>[12x]MAITPEQIAVEYPIPTYRFVVSVGDEQIPFNNVSGLDVHYDVIEYKDGIGNYYKMPGQRQSINITLRKGVFPGDTKLFDWINSIQLNQVEKKDIAISLTNEAGTEILMTWNVANAFPTSFTSPSFDATSNEIAVQEIALTADRVTIQAA;>MTTIT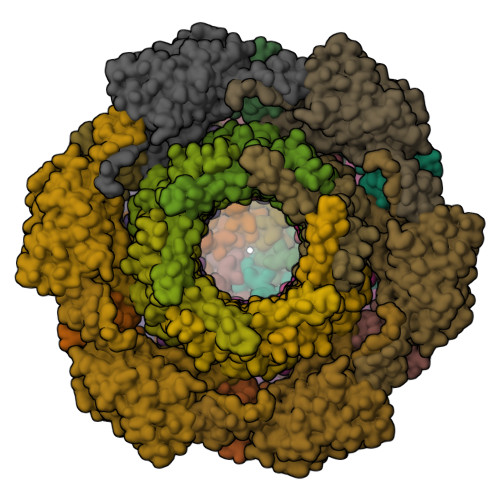TYPGVYIEEDASLSLSVSSSATAVPVFAVAGDNPLISGKPYIRISNWLEYLTLKNEQFDPANTLDISLRAYFINGGGYCYLVQTTDLEKQVPKLDDVTLLVAAGENITTAVSTLCKPGKGLFAIFDGPTTELKSDGTSNSDYDPNPFAAVYYPWLTADWTTTIDIPPSAAIAGVYCSVDSTRGVWKAPANVPIQGGLQPKYPVTDDLQAQYNQGKALNMIRTFPKSGTLVWGARTLEDNDNWRYIPVRRLFNSAERDIKNAMSFAVFEPNSQPTWERVRSAVNNYLYSLWQQGGLAGNKPDDAYFVQIGKDITMTDDDIKQGKMIIKIGMAAVRPAEFIILQFTQNTAQ[6x];>[6x]MTIIIASDNAIIEINQALNTILSQYLNITGQNIDIRFDLPEINSIQSEPTVSVFLYEIHEDLQLRSAESRRYNPSTNTLLPGWVNINCNYLITYWDASKPSSDSSSPDSQPNNQAAQVMTRILNALINNRQLTGLPGAYTRIIPQQENLNSLGNFWQALGNRPRLSLLYSITVPMKLKNIEDNVIPVSKISASVDQKPNLDNSQINQALIDKLCVELGGTEDVRLALAKVNLTTKPDTENNQNQENESVIVEVSGITSVTYLPQIKDTLTKWKSSQEAIVKINGVSIVVSKENADKLIGI>[18x]MSKSDVFHLGLTKNDLQGATLAIVPGDPDRVEKIAALMDKPVKLASH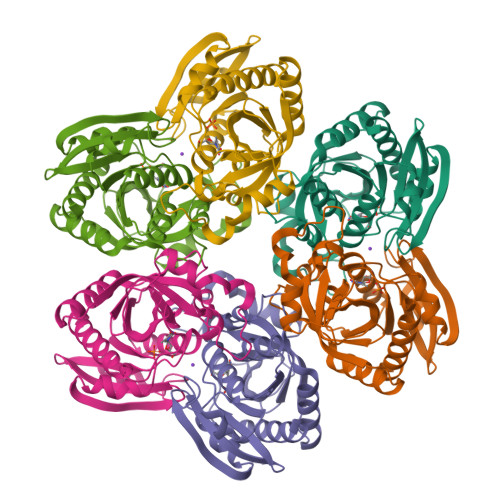REFTTWRAELDGKPVIVCSTGIGGPSTSIAVEELAQLGIRTFLRIGTTGAIQPHINVGDVLVTTASVRLDGASLHFAPLEFPAVADFECTTALVEAAKSIGATTHVGVTASSDTFYPGQERYDTYSGRVVRHFKGSMEEWQAMGVMNYEMESATLLTMCASQGLRAGMVAGVIVNRTQQEIPNAETMKQTESHAVKIVVEAARRLL>[3x]MTENAEKFLWGVATSAYQIEGATQEDGRGPSIWDAFAQRPGAIRDGSTGEPACDHYRRYEEDIALMQSLGVRAYRFSVAWPRILPEGRGRINPKGLAFYDRLVDRLLASGITPFLTLYHWDLPLALEERGGWRSRETAFAFAEYAEAVARALADRVPFFATLNEPWCSAFLGHWTGEHAPGLRNLEAALRAA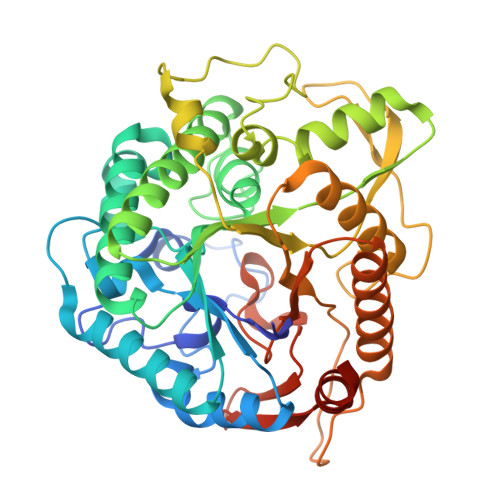HHLLLGHGLAVEALRAAGARRVGIVLNFAPAYGEDPEAVDVADRYHNRFFLDPILGKGYPESPFRDPPPVPILSRDLELVARPLDFLGVTYYAPVRVAPGTGTLPVRYLPPEGPATAMGWEVYPEGLHHLLKRLGREVPWPLYVTENGAAYPDLWTGEAVVEDPERVAYLEAHVEAALRAREEGVDLRGYFVWSLMDNFEWAFGYTRRFGLYYVDFPSQRRIPKRSALWYRERIARAQTHHHHHH(2S,5R,6R)-6-AMINO-3,3-DIMETHYL-7-OXO-4-THIA-1-AZABICYCLO[3.2.0]HEPTANE-2-CARBOXYLIC 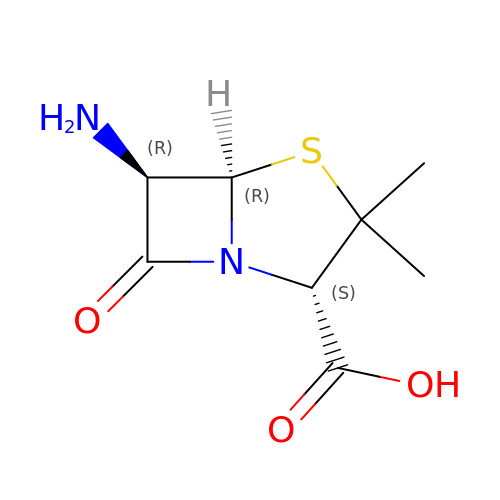ACID | C8 H12 N2 O3 S | NGHVIOIJCVXTGV-ALEPSDHESA-N>SMLKYSTNMLELAMPKINKIVNGTDLTPHYLSEPNKEFKIYRYNNEVYAVRFENDEPMDYVLMWKSHKSEHTQNSEMIKNTEEDYKELGKGEQGTVYEKTEDKAMKVSRGRHPREFYEEINLHIIEQQFFLKYHGIQEHFVLGLWNIKNEENVYFYMPKINAIPINKKIDQPKIEEFVLALKELNDAGYWHPDLANNPYHISPQNLIATEEMVKTIDLDGGFRYDKGRVDELSRKSLVYGKDQWLYVYNFIYPPTDEEDHRIDWRVPIEKWYE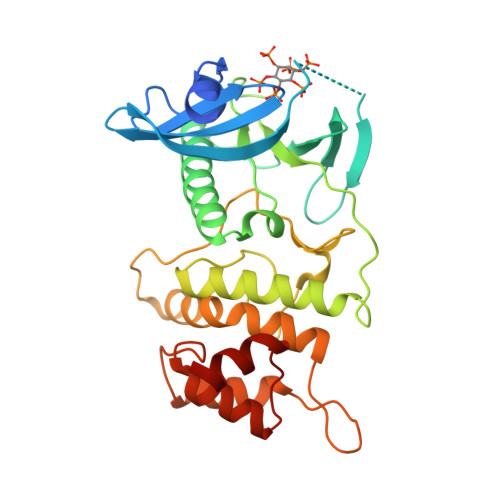NNRDESLSDNPHTLLRFYHEGLISLPKKLAHDLHETILEEL[3x]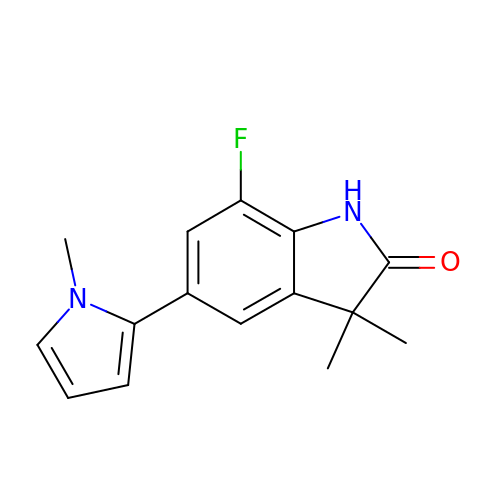7-fluoranyl-3,3-dimethyl-5-(1-methylpyrrol-2-yl)-1H-indol-2-one | C15 H15 F N2 O | HNCQSUFMNDUIEX-UHFFFAOYSA-N> MKIGIIGATGRAGSRILEEAKNRGHEVTAIVRNAGKITQTHKDINILQKDIFDLTLSDLSDQNVVVDAYGISPDEAEKHVTSLDHLISVLNGTVSPRLLVVGGAASLQIDEDGNTLLESKGLREAPYYPTARAQAKQLEHLKSHQAEFSWTYISPSAMFEPGERTGDYQIGKDHLLFGSDGNSFISMED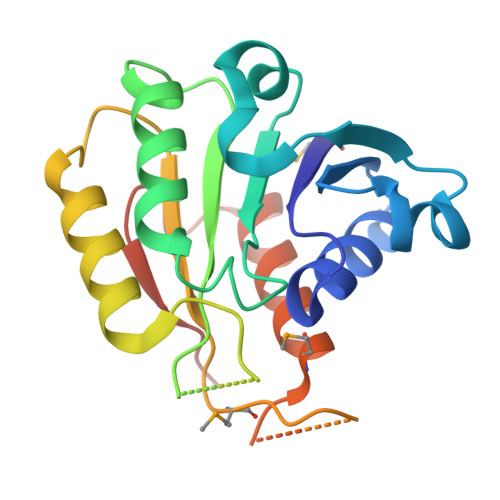YAIAVLDEIERPNHLNEHFTVAGKLEHHHHHH> 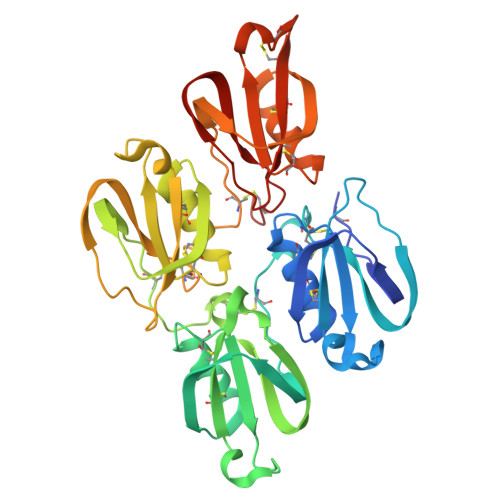RSHHHHHHGCLTQLYENAFFRGGDVASMYTPNAQYCQMRCTFHPRCLLFSFLPASSINDMEKRFGCFLKDSVTGTLPKVHRTGAVSGHSLKQCGHQISACHRDIYKGVDMRGVNFNVSKVSSVEECQKRCTNNIRCQFFSYATQTFHKAEYRNNCLLKYSPGGTPTAIKVLSNVESGFSLKPCALSEIGCHMNIFQHLAFSDVDVARVLTPDAFVCRTICTYHPNCLFFTFYTNVWKIESQRNVCLLKTSESGTPSSSTPQENTISGYSLLTCKRTLPEPCHSKIYPGVDFGGEELNVTFVKGVNVCQETCTKMIRCQFFTYSLLPEDCKAEACKCFLRLSMDGSPTRIAYGTQGSSGYSLRLCNTG> MVYQRQFLPADDRVTKNRKKVVDPSVKLEKIRTLSDKDFLTLIGHRHLGEAYRSVNPPLAEIGEPEDPIRELVPPTEGAKAGDRVCTIIMTDSVYNPPIAHYTRAWMYHNRFRGIDNGVYSGRVTLEMRERDLEEACRTLFETEICDASRDQVRQYTCTGHSCRLDPDGMMFDPI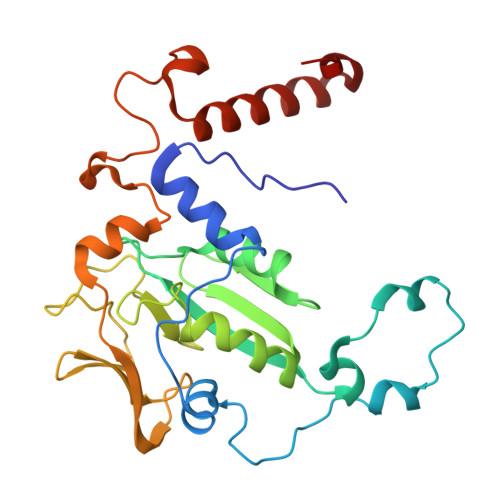ERCIMSGGNVVYQKDSFGNPVDTPINMGKPLSEEELIERTVVYRTDRGEPMTREGDPGAPDEEVREALQWSRRIQWLRMLGNMVPDKIKGM> DRIITDQLDRKVTIPDHINRAVVLQHQTLNIAVQLDATKQIVGVLSNWKKQLGKNYVRLAPELENMAMPGDLNSVNIESLLA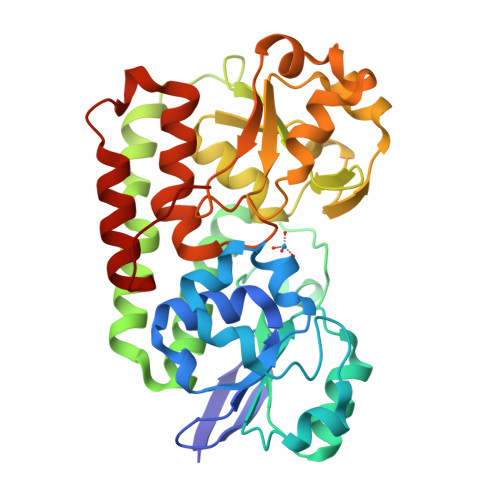LKPDVVFVTNYAPSEMIKQISDVNIPVVAISLRTGEVGEKGKLNPTLTDEDKAYNDGLKQGIELIAEVFEKKQQGDELVKAAFANRKLLADRLGDVSADKRVRTYMANPDLGTYGSGKYTGLMMEHAGAYNVAAATIKGFKQVSLENVLEWNPAVILVQDRYPDVVPQILNDQGWANIQALKDKKVFLMPEYAKAWGYPMPEALALGEVWLAKALYPQRFQDVDLDKMVNDYYQKFYRTSYKPD>MNKDLKGLYAALLVPFDENGQVNEQGLKQIAQNAIETEELDGLYVNGSSGENFLLNTEQKKQVFKVAKEAVGDKVKLIAQVGSLDLNEAIELGKYATELGYDALSAVTPFYYPFTFEEIRDYYFDIIEATQNNMIIYAIPDLTGVNISIEQFSELFNHEKIVGVKYTAPNFFLLERIRKAFPDKLILSGFDEMLVQATISGVDGAIGSTYNVNGRRARKIFDLARQGQIQEAYQLQHDSNDIIETVLSMGIYPTLKEILRH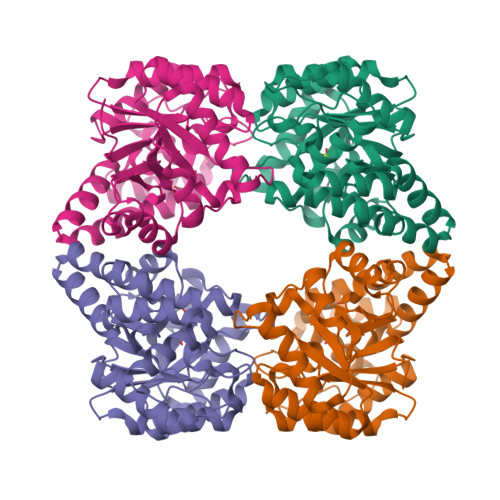RGIDAGLPKRPFKPFNEAHRQTLDQLIAKYDL[8x]>[2x]TTNKPIVLSTWNFGLHANVEAWKVLSKGGKALDAVEKGVRLVEDDPTERSVGYGGRPDRDGRVTLDACIMDENYNIGSVACMEHIKNPISVARAVMEKTPHVMLVGDGALEFALSQGFKKENLLTAESEKEWKEWLKTSQYKPIVNIENHDAIGMIALD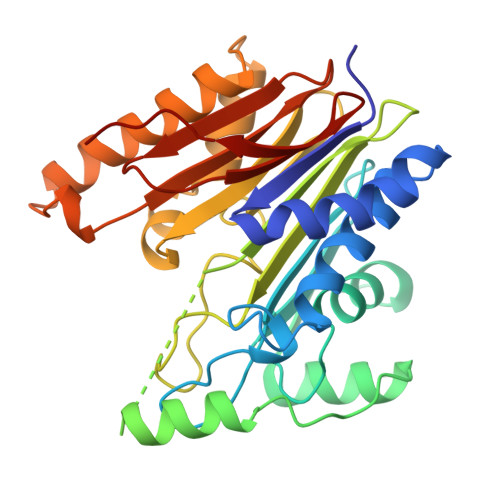AQGNLSGACTTSGMAYKMHGRVGDSPIIGAGLFVDNEIGAATATGHGEEVIRTVGTHLVVELMNQGRTPQQACKEAVERIVKIVNRRGKNLKDIQVGFIALNKKGEYGAYCIQDGFNFAVHDQKGNRLETPGFALK>GQDMVSPPPPIADEPLTVNTGIYLIESYSLDDCAETFKVNAFLSLSWKDRRLAFDPVRSGVRVKTYEPEAIWIPEIRFVNVENARDADVVDISVSPDGTVQYLERFSARVLSPLDFRRYPFDSQTLHIYLIVRSVDTRNIVLAVDLEKVGKNDDVFLTGWDIESFTAVVKPANFALEDRLESKLDYQLRISR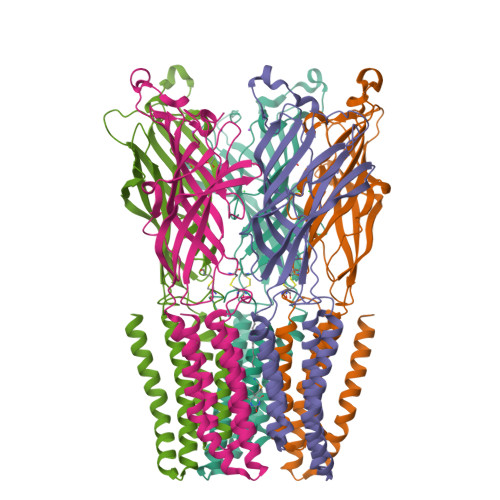QYFSYIPNIILPMLFILFISWTAFWSTSYEANVTLVVSTLIAHIAFNILVETNCPKTPYMTYTGAIIFMIYLFYFVAVIEVTVQHYLKVESQPARAASITRASRIAFPVVFLLANIILAFLFFGF[5x]>[2x]SSNDNIELVDFQNIMFYGDAEVGDNQQPFTFILDTGSANLWVPSVKCTTAGCLTKHLYDSSKSRTYEKDGTKVEMNYVSGTVSGFFSKDLVTVGNLSLPYKFIEVIDTNGFEPTYTASTFDGILGLGWKDLSIGSVDPIVVELKNQNKIENALFTFYLPVHDKHTGFLTIGGIEERFYEGPLTYEKLNHDLYWQITLDAHVGNIMLEK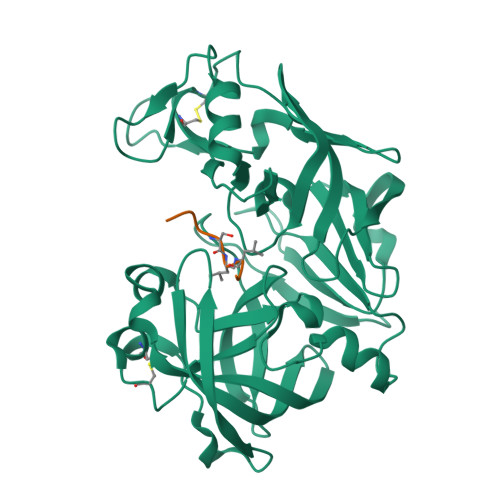ANCIVDSGTSAITVPTDFLNKMLQNLDVIKVPFLPFYVTLCNNSKLPTFEFTSENGKYTLEPEYYLQHIEDVGPGLCMLNIIGLDFPVPTFILGDPFMRKYFTVFDYDNHSVGIALAKKNL;>KPFSXLQF[2x]>[12x]MAHHHHHHMIPKTMKAAVVQGYGEPLKIQEVPVREPGRYEVLVKVMACGVC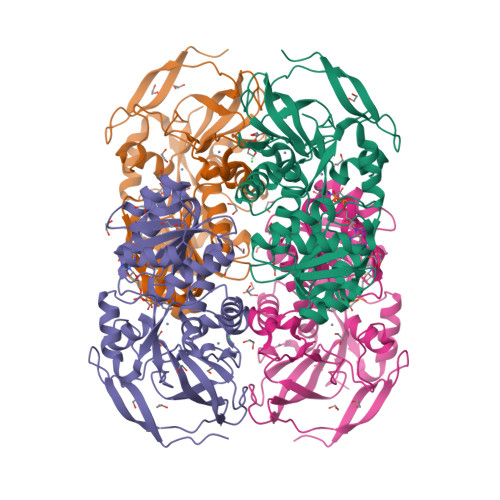HTDLHAVDGDWPAKPKMPLIPGHEGVGIVVACGPDAMVKEGDAVGVPWLYSACGCCDYCITGWETLCEAQQNGGYSVDGGFAEYVIADSRYVGHLKSNVNFLEIAPILCAGVTVYKGLKETETKPGEWVAISGIGGLGHVAVQYAKAMGMHVAAIDVADDKLELAKKLGADLTVNAKTTDPGTYLHKEVGGMHGALITAVSPIAFKQGIDVLRRKGTIALNGLPPGSFELPIFETVLKRITVRGSIVGTRKDLQEALDFANEGLVKATVTSAKLEDINDVFDKMKKGQIDGRIVLDIAGSQN>[2x]MGSDKIHHHHHHMKVIETKYSGKLEVAEDRLIAFDQGIPAFEDEKEFVLLPFAAGTPYYT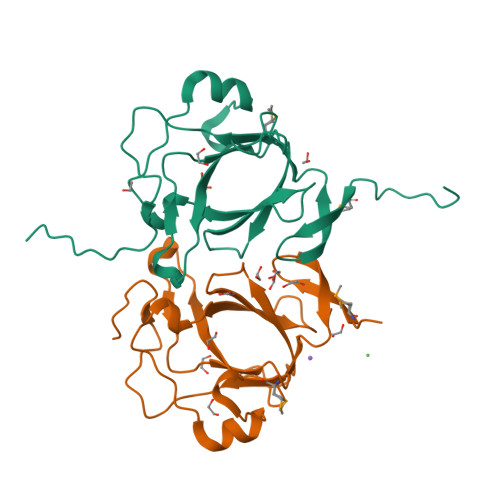LQSTKTVDLAFIIVNPFSFFPEYRVKLPEATIAQLNITNENDVAIFSLLTVKEPFSETTVNLQAPIVINANKQMGKQLVLGDTAYNRKQPLFQKELVLAKEAK>[2x]GAMAGDQELELRFDVPLYTLAEASRYLVVPRATLATWADGYERRPANAPAVQGQPIITALPHPTGSHARLPFVGIAEAYVLNAFRRAGVPM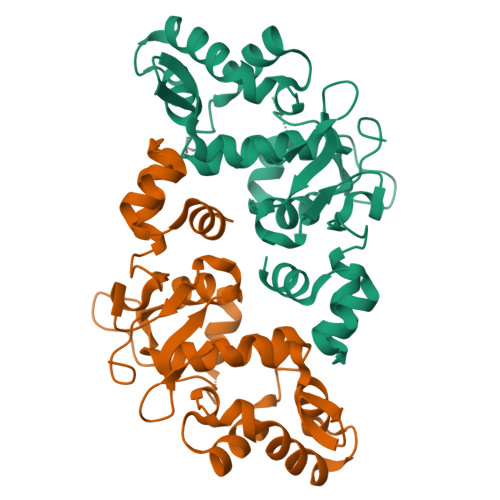QRIRPSLDWLIKNVGPHALASQDLCTDGAEVLWRFAERSGEGSPDDLVVRGLIVPRSGQYVFKEIVEHYLQQISFADDNLASMIRLPQYGDANVVLDPRRGYGQPVFDGSGVRVADVLGPLRAGATFQAVADDYGVTPDQLRDALDAIAA Defense-associated sirtuin 2 (DSR2) systems are widely distributed across prokaryotic genomes, providing robust protection against phage infection. DSR2 recognizes phage tail tube proteins and induces abortive infection by depleting intracellular NAD+, a process that is counteracted by another phage-encoded protein, DSR Anti Defense 1 (DSAD1). Each DSR2 protomer consists of a conserved N-terminal Sirtuin (SIR2) domain, a C-terminal domain (CTD) and a middle domain (MD). DSR2 assembles into an elongated tetramer, with four NADase catalytic modules clustered in the center and the regulatory-sensing modules distributed at four distal corners.

Here, we collected high-quality cryo-EM data to generate a three-dimensional map of the DSR2-DSAD1 complex with a nominal resolution of 3.49 Å, providing detailed information on the complex architecture and functional insights. The structure shows that DSAD1 binds directly to the CTD of DSR2 at the site typically used for Tube binding and activation of DSR2. Structure and sequence alignments show that the inhibitory DSR2-DSAD1 complex cannot bind to the phage tube protein due to a steric clash between two proteins at the binding interface. Our results demonstrate that DSAD1 competes with Tube for the binding site of DSR2, resulting in the inhibition of DSR2 activation by Tube. The DSAD1 protein and DSR2 assemble in a 2:4 ratio, forming an inhibited state. Each X-shaped DSR2 dimer interacts with one DSAD1 protein. The interactions between DSR2 and DSAD1 are mainly contributed by hydrophobic interactions (F59 of DSAD1 to I918/W919/L922/Y962/L966 of DSR2(a)) and further strengthened by hydrogen bonds (S107/S108 of DSAD1 to S957/N961 of DSR2(a)). There is also an additional hydrophobic interaction between DSAD1 and the opposite DSR2 (L14/V15/Y16 of DSAD1 to F576/Y574 of DSR2(b)). Furthermore, the DSR2-DSAD1 tetramer in the inhibited state shows a structure similar to the “loose” conformation observed in the inactive apo DSR2 tetramer. In contrast, binding of the inhibitor DSAD1 to DSR2 induced minor conformational changes in DSR2.

>[4x]VKVDLESKRYGEKLKEVFLMLDNNVVECIKEITESSRNGKLVFFVGAGVSTLSDYPQWWRLVDKYHEELYGSPKKGNYSSDEYLRIPQIFYNVKGEMAFDGILKDFFQVDKPTNPIHDKILAMNPAHVITTNYDNLIDTACWKRGKYFSVISAEEDVANATSSRYLLKVHGDFRKGFKGENVVLKEDDYLNYDQNYPLISNLMKTIIATHTIVFIGYGLGDYNINMLLNWVRKLQKDSFHKPFFIRTDPSPIENETLIYYENKGLRIIDAASLIDSNEYDYLERYSAVMDLLIESQENKFITKDDEVIDYIYGKISPLFALQYIRKIDLKHVFEYDYHFEVNGTVVRHKNKGFGYMERFFELKESCDERSKLSKKQYERFNALFNFFEKNGVICMAKDAGTLNTSIEINSLAYHGKYDVMKKFIEEQSVSIEDDYKKAFFLACLGRWEESYDLYSNIILNSIDESNGCVYYLSQINRYRIYQSITQAVTQFNGLGLLTFGRHYKPFTDEFLARIEREMTNFNIDDLFNGMPFEFQKKYKILEFLSDNQFLYDDTVKLFELTNKVRSEMSEGSYSFGMSSDIVVLLRLYDNLRFLYENCLWSVSFHEFHQYIRNSMSLLIEKAEYERTRDIDELGFSFFGKKSGFFMEYYDFVNISRHFKIDDIKNLERSCSIDKIRFGEQEKIEEYLVGIAEEITKQFSANGMNVVFYTQFISEAKAALYFAKYVKLSEEGLGKIVKALLFYFPERDLDIGKRYVWLERLTKCNELPKSIISIIDDFLVLQAEKHIDQNYSEVSSNGLYSRDYGALIKHFEKNFISKRLSEITLCLTQDKQKQIDFLFKLLPLLSTNAKSHLLSFKSVENINDLMNGIRIGLIDEFTPEHEELIIEYLETRKVNYIVEKEKGIQTFSSNDYMSTFGIWYFLEEINNSKMEEFIGMDDQYDFFVDPENFDYKKFIPSWLKNYNDKLLGKIAGNKHMKHHVIEVLKERVKNSNDKRYLEILMNYFI;> MIEIFKDTGATHDLVYHSKINTFVWDVEFDIVLSDSKELNKCYFVKCFNPYRINGKCDFAVSSIDIFSEGKRLLIENEFNFKITKAVHVATSKDVTEIVLHLSERISSPFPIVKEVVYLD>[8x]MKKWVCTVCGYIYDEDAGDPDNGISPGTKFEELPDDWVCPLCGVGKDQFEKLED

Chimeric hybrids derived from the rubredoxins of Pyrococcus furiosus (Pf) and Clostridium pasteurianum (Cp) provide a robust system for the characterization of protein conformational stability and dynamics in a differential mode. A structure design algorithm was applied to the rubredoxins from Pyrococcus furiosus and the mesophilic bacterium Clostridium pasteurianum (Cp) to generate chimeric proteins in which the predicted hybridization interface can preserve each of the interactions in the parental structures. Interchange of the seven nonconserved residues in the metal binding site region between the Cp and Pf A2K rubredoxins yields two complementary hybrid proteins that are accurately represented as a sum of segments from the parental structures. These "cut-and-paste" models match the ultra-high resolution X-ray models to within the structural variability exhibited by the crystallographically nonequivalent molecules in the unit cell.

The metal binding site-swapped Pf A2K rubredoxin crystallized at pH 5.5 in a P21 space group, with eight molecules per asymmetric unit. In contrast, the P212121 crystals used to determine the Pf rubredoxin structure formed at pH 8.5, with a single molecule in the asymmetric unit. The refinement for all reflections out to 1.04 Å, utilizing anisotropic B-factors and all hydrogens, yielded a final R (Rfree) factor of 13.9% (18.0%). The asymmetric unit is arranged as four pairs of dimers. Residues 20–23 from molecules A-D form an asymmetric interaction with the corresponding loop residues of their dimer partners of molecules E-H. All of the first four molecules of the asymmetric unit agree with one another to within less than 0.3 Å for all sidechain and mainchain heavy atoms, when residues 20–26 are excluded. Despite the differences in sequence, space group and pH conditions, the backbone coordinates of molecule A differ from those of the original search model by an rmsd value of only 0.22 Å, with modestly larger values for Molecules B, C and D. In contrast, the deviations from the backbone coordinates of the search model were approximately 0.6 Å larger for molecules E-H. For Molecules A to D of the metal binding site-swapped Pf A2K rubredoxin, sidechains exhibiting dual conformations are Ser 25, Val 44 and Gln 48. The interactions of the three charged residues Lys 29, Glu 31 and Glu 32 vary substantially among the molecules of the asymmetric unit, with the Lys 29 sidechain exhibiting weak electron density. Relative to the X-ray structure, the NMR-derived structure adopts a differing χ1 dihedral angle for Asp 47 and χ2 for Glu 50. The Asp 35 sidechain of the metal binding site-swapped Pf A2K rubredoxin X-ray structure is rotated out toward the solvent phase, away from the Lys 46 Nζ atom, consistent with the findings of the NMR analysis.> ERAAKCRAYAKALHYKELEFQKGPTPAILESLISINNKLQQPEAAAGVLEYAMKHFGELEIQATWYEKLHEWEDALVAYDKKMDTNKDDPELMLGRMRCLEALGEWGQLHQQCCEKWTLVNDETQAKMARMAAAAAWGLGQWDSMEEYTCMIPRDTHDGAFYRAVLALHQDLFSLAQQCIDKARDLLDAELTAMAGESYSRAYGAMVSCHMLSELEEVIQYKLVPERREIIRQIWWERLQGCQRIVEDWQKILMVRSLVVSPHEDMRTWLKYASLCGKSGRLALAHKTLVLLLGVDPSRQLDHPLPTVHPQVTYAYMKNMWKSARKIDAFQHMQHFVQTMQQQAQHAIATEDQQHKQELHKLMARCFLKLGEWQLNLQGINESTIPKVLQYYSAATEHDRSWYKAWHAWAVMNFEAVLHYKHQNQARDEKKKLRHASGANITNATTAATTAATATTTASTEGSNSESEAESTENSPTPSPLQKKVTEDLSKTLLMYTVPAVQGFFRSISLSRGNNLQDTLRVLTLWFDYGHWPDVNEALVEGVKAIQIDTWL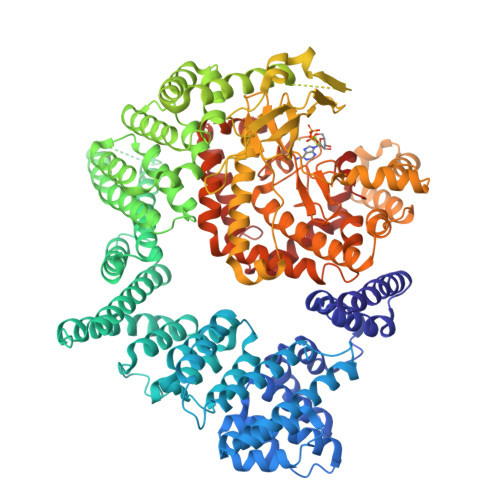QVIPQLIARIDTPRPLVGRLIHQLLTDIGRYHPQALIYPLTVASKSTTTARHNAANKILKNMCEHSNTLVQQAMMVSEELIRVAILWHEMWHEGLEEASRLYFGERNVKGMFEVLEPLHAMMERGPQTLKETSFNQAYGRDLMEAQEWCRKYMKSGNVKDLTQAWDLYYHVFRRISKQLPQLTSLELQYVSPKLLMCRDLELAVPGTYDPNQPIIRIQSIAPSLQVITSKQRPRKLTLMGSNGHEFVFLLKGHEDLRQDERVMQLFGLVNTLLANDPTSLRKNLSIQRYAVIPLSTNSGLIGWVPHCDTLHALIRDYREKKKILLNIEHRIMLRMAPDYDHLTLMQKVEVFEHAVNNTAGDDLAKLLWLKSPSSEVWFDRRTNYTRSLAVMSMVGYILGLGDRHPSNLMLDRLSGKILHIDFGDCFEVAMTREKFPEKIPFRLTRMLTNAMEVTGLDGNYRITCHTVMEVLREHKDSVMAVLEAFVYDPLLNWRLMDTNTKGNKRSRTRTDSYSAGQSVEILDGVELGEPAHKKTGTTVPESIHSFIGDGLVKPEALNKKAIQIINRVRDKLTGRDFSHDDTLDVPTQVELLIKQATSHENLCQCYIGWCPFW> MSATKSIVGEALEYVNIGLSHFLALPLAQRISLIIIIPFIYNIVWQLLYSLRKDRPPLVFYWIPWVGSAVVYGMKPYEFFEECQKKYGDIFSFVLLGRVMTVYLGPKGHEFVFNAKLADVSA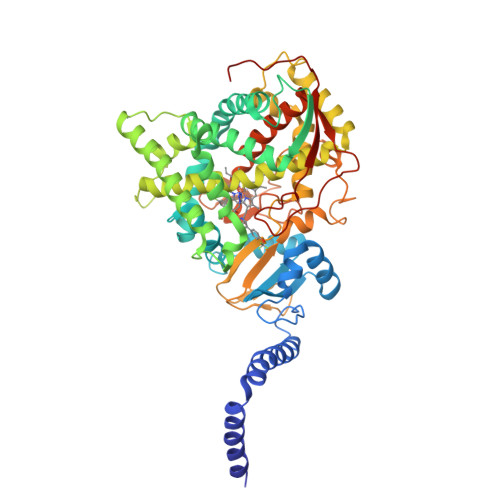EAAYAHLTTPVFGKGVIYDCPNSRLMEQKKFVKGALTKEAFKSYVPLIAEEVYKYFRDSKNFRLNERTTGTIDVMVTQPEMTIFTASRSLLGKEMRAKLDTDFAYLYSDLDKGFTPINFVFPNLPLEHYRKRDHAQKAISGTYMSLIKERRKNNDIQDRDLIDSLMKNSTYKDGVKMTDQEIANLLIGVLMGGQHTSAATSAWILLHLAERPDVQQELYEEQMRVLDGGKKELTYDLLQEMPLLNQTIKETLRMHHPLHSLFRKVMKDMHVPNTSYVIPAGYHVLVSPGYTHLRDEYFPNAHQFNIHRWNNDSASSYSVGEEVDYGFGAISKGVSSPYLPFGGGRHRCIGEHFAYCQLGVLMSIFIRTLKWHYPEGKTVPPPDFTSMVTLPTGPAKIIWEKRNPEQKIGGRHHH>MATTIKENEFLCDEEIYKSFVHLKDKICEERKKKELVSYSSYIKEMKKLLKVVLLKYKALKFGEFILKSKRKSNYFFSSGVLNNIVSSNIICFLLSELILKNKLSFDYLLGASYKGIPMVSLTSHFLFESKKYSNIFYLYDRKEKKEYGDKNVIVGNLDDDDKDILNLKKKTKNNQDEEKKNIIIIDDVFTCGTALTEILAKLKTYEHLKVVAFIVLLNRNEYEINENNQKIYFKDIFEKRVGIPLYSILSYKDDIQSMIHHHHHH[8x]

Specifically, P. falciparum orotate phosphoribosyltransferase (PfOPRTase), the fifth enzyme in the indispensible de novo pyrimidine-synthesis pathway of the parasite, is of special interest. OPRTase catalyses the conversion of orotate and 5-phospho-d-ribosyl 1-pyrophosphate (PRPP) into orotidine 5′-monophosphate (OMP). OPRTase is a dimeric enzyme with two active-site pockets, one on each protomer. Once the substrate has docked, two different loops, one from each protomer, cover the bound substrate to shield it from solvent.

In our crystal, PfOPRTase 1–218(Δ37–58)-H6 packs as a set of four catalytic dimers, leading to eight molecules in the asymmetric unit. In the present crystal, the individual PfOPRTase molecules possess the conserved α/β topology also seen in other OPRTases. The PfOPRTase structure conforms with the conserved PRTase fold, having a 321456 arrangement of β-sheets. There are 2–6 sulfate ions originating from the crystallization conditions associated with each polypeptide in the core dimer. The two most interesting sulfate ions occupy the positions where the phosphate and pyrophosphate groups of the PRPP substrate are expected to bind. Remarkably, of the 11 active-site residues at the core of the human enzyme, five are different in the malarial enzyme. In this larger tetrameric structure, a protomer from one catalytic dimer forms an inhibitory interaction with the active site of another protomer but from a different neighboring catalytic dimer. A β-hairpin formed by β8 and β9 (243EYEINENNQKIY254) inserts itself exactly at the substrate-binding pocket of the recipient active site. This completely occludes the closure of the hood domain and would prevent crucial substrate interactions, including π-stacking with Phe97, in the hood domain. Presumably, these intersubunit interactions blocking the active site of PfOPRTase occurred at high crystallization concentrations, but they hint at protein–protein interactions leading to autologous catalytic inhibition of PfOPRTase that may regulate flux through this enzyme.(1R,3R,7E,17Z)-17-(5-hydroxy-1,5-dimethylhexylidene)-2-methylene-9,10-secoestra-5,7-diene-1,3-diol | C27 H42 O3 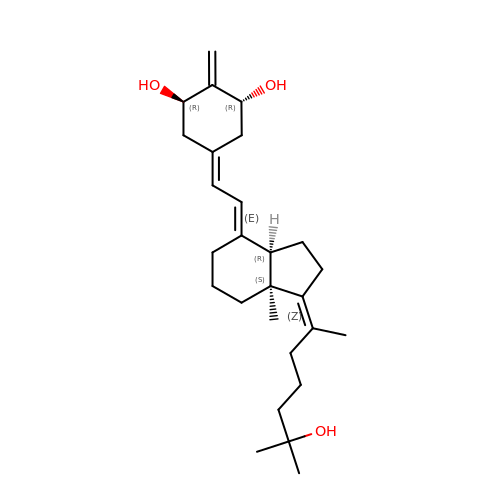| PCPYFQNISYYIPU-DUKKOGHCSA-N>[2x]MVGGGGVKFIEMDIRDKEAYELAKEWFDEVVVSIKFNEEVDKEKLREARKEYGKVAILLSNPKPSLVRDTVQKF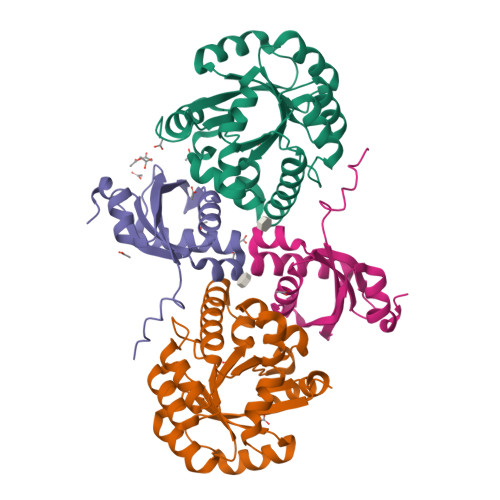KSYLIYVESNDLRVIRYSIEKGVDAIISPWVNRKDPGIDHVLAKLMVKKNVALGFSLRPLLYSNPYERANLLRFMMKAWKLVEKYKVRRFLTSSAQEKWDVRYPRDLISLGVVIGMEIPQAKASISMYPEIILKRLKY;>[2x]MMRKLKTLPPTLRDKNRYIAFEIISDGDFTKDEVKELIWKSSLEVLGETGTAIVKPWLIKFDPNTKTGIVRSDREYVEYLRFALMLVSEFNGKRLIIRTLGVSGTIKRLKRKFLAKYGWK>[2x]DMEIACLDLEGVLVPEIWIAFAEKTGIDALKATTRDIPDYDVLMKQRLRILDEHGLKLGDIQEVIATLKPLEGAVEFVDWLR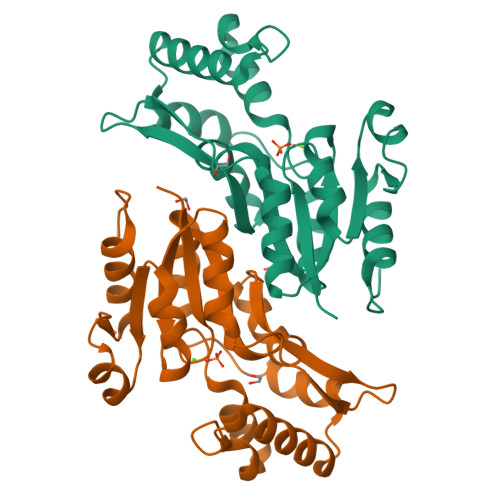ERFQVVILSDTFYEFSQPLMRQLGFPTLLCHKLEIDDSDRVVGYQLRQKDPKRQSVIAFKSLYYRVIAAGDSYNDTTMLSEAHAGILFHAPENVIREFPQFPAVHTYEDLKREFLKASSRSLSL[(3~{R})-3-carboxy-7-[(2,3-dimethylphenyl)methyl]-5-oxidanylidene-2,3-dihydro-[1,3]thiazolo[3,2-a]pyridin-8-yl]-dimethyl-azanium | C19 H23 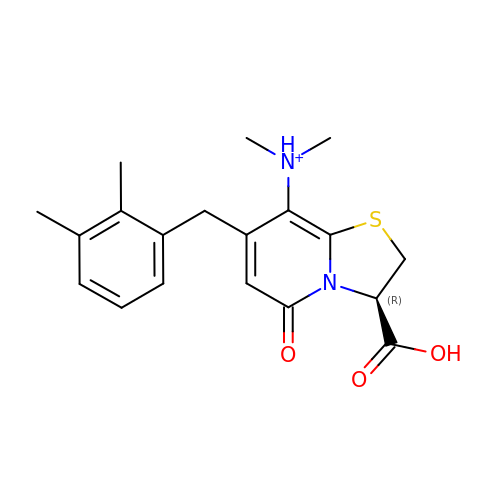N2 O3 S | ROYOKFGWFIQXTM-HNNXBMFYSA-O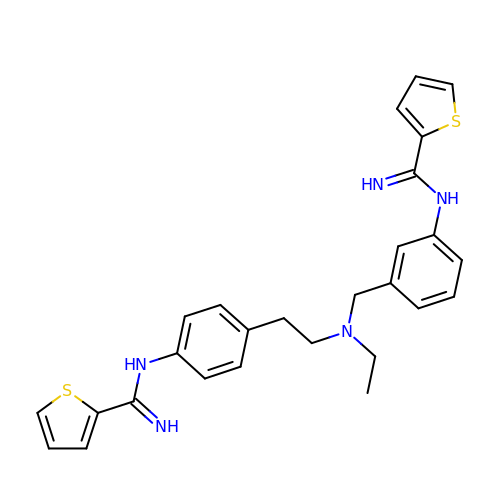N-(4-{2-[ethyl(3-{[(E)-imino(thiophen-2-yl)methyl]amino}benzyl)amino]ethyl}phenyl)thiophene-2-carboximidamide | C27 H29 N5 S2 | ZAOJVZLLICOZMJ-UHFFFAOYSA-N>MLDSKLKAPVFTVRTQGREYGEFVLEPLERGFGVTLGNPLRRILLSSIPGTAVTSVYIEDVLHEFSTIPGVKEDVVEIILNLKELVVRFLNPSLQTVTLLLKAEGPKEVKARDFLPVADVEIMNPDLHIATLEEGGRLNMEVRVDRGVGYVPAEKHGIKDRINAIPVDAVFSPVRRVAFQVEDTRLGQRTDLDKLTLRIWTDGSVTPLEALNQAVEILREHLTYFSNPQAAAVAAPEEAKEPEAPPEQEEELDLPLEELGLSTRVLHSLKEEGIESVRALLALNLKDLKNIPGIGERSLEEIKEALEKKGFTLKE[2x];> MEIKRFGRIREVIPLPPLTEIQVESYRRALQADVPPEKRENVGIQAAFRETFPIEEEDKGKGGLVLDFLEYRLGEPPFPQDECREKDLTYQAPLYARLQLIHKDTGLIKEDEVFLGHIPLMTEDGSFIINGADRVIVSQIHRSPGVYFTPDPARPGRYIASIIPLPKRGPWIDLEVEPNGVVSMKVNKRKFPLVLLLRVLGYDQETLARELGAYGELVQGLMDESVFAMRPEEALIRLFTLLRPGDPPKRDKAVAYVYGLIADPRRYDLGEAGRYKAEEKLGIRLSGRTLARFEDGEFKDEVFLPTLRYLFALTAGVPGHEVDDIDHLGNRRIRTVGELMTDQFRVGLARLARGVRERMLMGSEDSLTPAKLVNSRPLEAAIREFFSRSQLSQFKDETNPLSSLRHKRRISALGPGGLTRERAGFDVRDVHRTHYGRICPVETPEGANIGLITSLAAYARVDELGFIRTPYRRVVGGVVTDEVVYMTATEEDRYTIAQANTPLEGNRIAAERVVARRKGEPVIVSPEEVEFMDVSPKQVFSVNTNLIPFLEHDDANRALMGSNMQTQAVPLIRAQAPVVMTGLEERVVRDSLAALYAEEDGEVAKVDGNRIVVRYEDGRLVEYPLRRFYRSNQGTALDQRPRVVVGQRVRKGDLLADGPASENGFLALGQNVLVAIMPFDGYNFEDAIVISEELLKRDFYTSIHIERYEIEARDTKLGPERITRDIPHLSEAALRDLDEEGVVRIGAEVKPGDILVGRTSFKGESEPTPEERLLRSIFGEKARDVKDTSLRVPPGEGGIVVRTVRLRRGDPGVELKPGVREVVRVYVAQKRKLQVGDKLANRHGNKGVVAKILPVEDMPHLPDGTPVDVILNPLGVPSRMNLGQILETHLGLAGYFLGQRYISPIFDGAKEPEIKELLAQAFEVYFGKRKGEGFGVDKREVEVLRRAEKLGLVTPGKTPEEQLKELFLQGKVVLYDGRTGEPIEGPIVVGQMFIMKLYHMVEDKMHARSTGPYSLITQQPLGGKAQFGGQRFGEMEVWALEAYGAAHTLQEMLTLKSDDIEGRNAAYEAIIKGEDVPEPSVPESFRVLVKELQALALDVQTLDEKDNPVDIFEGLASKR;> MKKEVRKVRIALASPEKIRSWSYGEVEKPETINYRTLKPERDGLFDERIFGPIKDYECACGKYKRQRFEGKVCERCGVEVTKSIVRRYRMGHIELATPAAHIWFVKDVPSKIGTLLDLSATELEQVLYFSKYIVLDPKGAILNGVPVEKRQLLTDEEYRELRYGKQETYPLPPGVDALVKDGEEVVKGQELAPGVVSRLDGVALYRFPRRVRVEYVKKERAGLRLPLAAWVEKEAYKPGEILAELPEPYLFRAEEEGVVELKELEEGAFLVLRREDEPVATYFLPVGMTPLVVHGEIVEKGQPLAEAKGLLRMPRQVRAAQVEAEEEGETVYLTLFLEWTEPKDYRVQPHMNVVVPEGARVEAGDKIVAAIDPEEEVIAEAEGVVHLHEPASILVVKARVYPFEDDVEVSTGDRVAPGDVLADGGKVKSDVYGRVEVDLVRNVVRVVESYDIDARMGAEAIQQLLKELDLEALEKELLEEMKHPSRARRAKARKRLEVVRAFLDSGNRPEWMILEAVPVLPPDLRPMVQVDGGRFATSDLNDLYRRLINRNNRLKKLLAQGAPEIIIRNEKRMLQEAVDALLDNGRRGAPVTNPGSDRPLRSLTDILSGKQGRFRQNLLGKRVDYSGRSVIVVGPQLKLHQCGLPKRMALELFKPFLLKKMEEKGIAPNVKAARRMLERQRDIKDEVWDALEEVIHGKVVLLNRAPTLHRLGIQAFQPVLVEGQSIQLHPLVCEAFNADFDGDQMAVHVPLSSFAQAEARIQMLSAHNLLSPASGEPLAKPSRDIILGLYYITQVRKEKKGAGLEFATPEEALAAHERGEVALNAPIKVAGRETSVGRLKYVFANPDEALLAVAHGIVDLQDVVTVRYMGKRLETSPGRILFARIVAEAVEDEKVAWELIQLDVPQEKNSLKDLVYQAFLRLGMEKTARLLDALKYYGFTFSTTSGITIGIDDAVIPEEKKQYLEEADRKLLQIEQAYEMGFLTDRERYDQILQLWTETTEKVTQAVFKNFEENYPFNPLYVMAQSGARGNPQQIRQLCGLRGLMQKPSGETFEVPVRSSFREGLTVLEYFISSHGARKGGADTALRTADSGYLTRKLVDVTHEIVVREADCGTTNYISVPLFQPDEVTRSLRLRKRADIEAGLYGRVLAREVEVLGVRLEEGRYLSMDDVHLLIKAAEAGEIQEVPVRSPLTCQTRYGVCQKCYGYDLSMARPVSIGEAVGIVAAQSIGEPGTQLTMRTFHTGGVAGAADITQGLPRVIELFEARRPKAKAVISEIDGVVRIEETEEKLSVFVESEGFSKEYKLPKEARLLVKDGDYVEAGQPLTRGAIDPHQLLEAKGPEAVERYLVEEIQKVYRAQGVKLHDKHIEIVVRQMMKYVEVTDPGDSRLLEGQVLEKWDVEALNERLIAEGKTPVAWKPLLMGVTKSALSTKSWLSAASFQNTTHVLTEAAIAGKKDELIGLKENVILGRLIPAGTGSDFVRFTQVVDQKTLKAIEEARKEAVEAKERPAARRGVKREQPGKQADYKDDDDK;> MAEPGIDKLFGMVDSKYRLTVVVAKRAQQLLRHGFKNTVLEPEERPKMQTLEGLFDDPNAVTWAMKELLTGRLVFGENLVPEDRLQKEMERLYPGEREE

Transcription termination is an essential step in transcription by RNA polymerase (RNAP) and crucial for gene regulation. For many bacterial genes, transcription termination is mediated by the adenosine triphosphate–dependent RNA translocase/helicase Rho, which causes RNA/DNA dissociation from the RNAP elongation complex (EC). Rho is an adenosine triphosphate (ATP)–dependent RNA translocase/helicase with 5′ → 3′ directionality. Rho forms a ring-shaped homo-hexameric complex, mediated by the CTD.

Cryo-EM maps of Rho, apo RNAP, EC, and type 1 and type 2 complexes are shown. For the cryo-EM analysis of the EC-Rho complex, the EC was prepared using the same DNA/RNA as in the RNA release assay. A 125-nucleotide RNA was elongated by adding ATP, cytidine triphosphate (CTP), and uridine triphosphate (UTP), and the EC was stalled at the first G stretch on the DNA. The EC holds a transcription bubble containing a 10-bp DNA/RNA hybrid within the RNAP main channel. The EC is stalled immediately before the G-triad of the template DNA.> MNDDAELYRNSSSMQRRDALNSL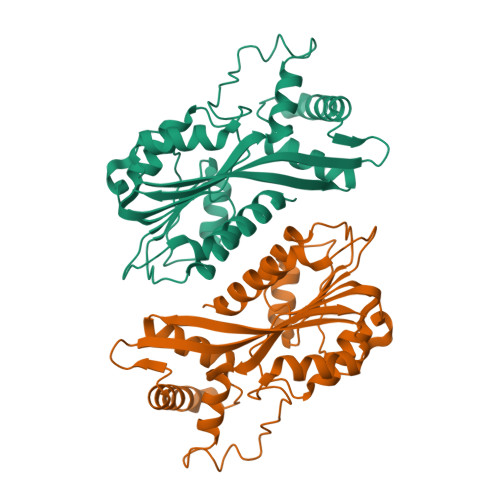TEYLPKFKWKESKEKILDIGCADGSVTNIISSCCPTDFELFEACDVNVKSVKYATEHYGTSKMRFRVMDIESDLPKEMKGKFDHVFSFYTLHWIENQEKAFQNIYDLTADDGECFLTLLAQMPVFNLFDALKHTEKWRHWLRYIKNFISPYYETSDPDVVIELLLKRVGFRYVDVRCRQKKFEFYDLKSFRNLLEAVSPFKVGQELQEELIDDVMEVAKEMRIIDTQNSTAKLIYNLVVIHCRK> PIETVPVKLKPGMDGPKVKQWPLTEEKIKALVEICTEMEKEGKISKIGPENPYNTPVFAIKKKDSTKWRKLVDFRELNKRTQDFWEVQLGIPHPAGLEKKKSVTVLDVGDAYFSVPLDEDFRKYTAF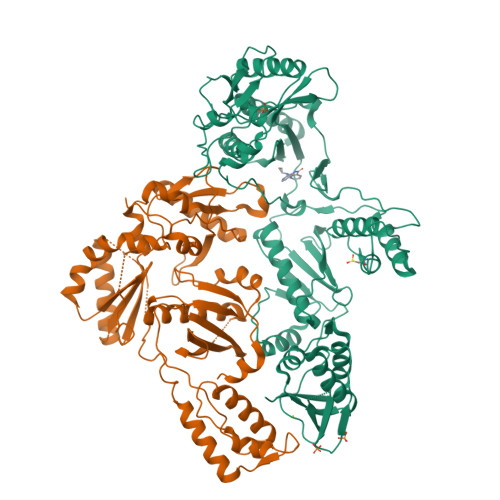TIPSINNETPGIRYQYNVLPQGWKGSPAIFQSSMTKILEPFRKQNPDIVIYQYMDDLYVGSDLEIGQHRTKIEELRQHLLRWGLTTPDKKHQKEPPFLWMGYELHPDKWTVQPIVLPEKDSWTVNDIQKLVGKLNWASQIYPGIKVRQLCKLLRGTKALTEVIPLTEEAELELAENREILKEPVHGVYYDPSKDLIAEIQKQGQGQWTYQIYQEPFKNLKTGKYARMRGAHTNDVKQLTEAVQKITTESIVIWGKTPKFKLPIQKETWETWWTEYWQATWIPEWEFVNTPPLVKLWYQLEKEPIVGAETFYVDGAANRETKLGKAGYVTNRGRQKVVTLTDTTNQKTELQAIYLALQDSGLEVNIVTDSQYALGIIQAQPDQSESELVNQIIEQLIKKEKVYLAWVP;> TVPVKLKPGMDGPKVKQWPLTEEKIKALVEICTEMEKEGKISKIGPENPYNTPVFAIKKKDSTKWRKLVDFRELNKRTQDFWEVQLGIPHPAGLEKKKSVTVLDVGDAYFSVPLDEDFRKYTAFTIPSINNETPGIRYQYNVLPQGWKGSPAIFQSSMTKILEPFRKQNPDIVIYQYMDDLYVGSDLEIGQHRTKIEELRQHLLRWGLTTPDKKHQKEPPFLWMGYELHPDKWTVQPIVLPEKDSWTVNDIQKLVGKLNWASQIYPGIKVRQLCKLLRGTKALTEVIPLTEEAELELAENREILKEPVHGVYYDPSKDLIAEIQKQGQGQWTYQIYQEPFKNLKTGKYARMRGAHTNDVKQLTEAVQKITTESIVIWGKTPKFKLPIQKETWETWWTEYWQATWIPEWEFVNTPPLVKLWYQ> GSHMASMKKKGSVVIVGRINLSGDTAYAQQTRGEEGCQETSQTGRDKNQVEGEVQIVSTATQTFLATSINGVLWTVYHGAGTRTIASPKGPVTQMYTNVDKDLVGWQAPQGSRSLTPCTCGSSDLYLVTRHADVIPVRRRGDSTGSLLSPRPLSYLKGSSGGPLLCPAGHAVGIFRAAVSTRGVAKAVQFIPVES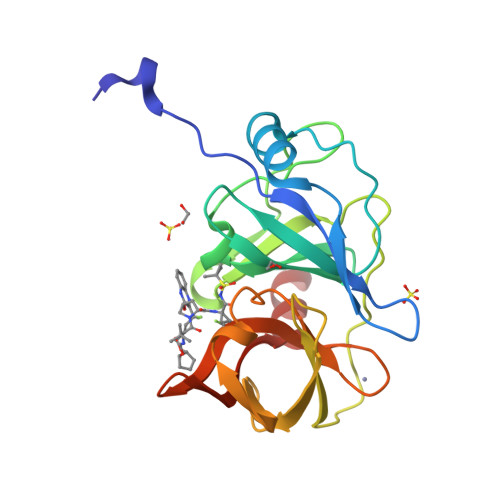LETTMRSP Briefly, this product is produced by a typical NRPS assembly line of four subunits: PchD, PchE, PchF, and PchG. PchD activates salicylate, PchE and PchF successively integrate two l-cysteines into the growing peptide to form two thiazoline rings, and PchG then reduces the second thiazoline ring to thiazolidine before the release of mature pyochelin. The adenylation domain (A) in PchE selects and activates l-cysteine; aryl carrier protein (ArCP) and peptidyl carrier protein (PCP) connect and transfer salicylate and l-cysteine using phosphopantetheine (pPant) arms, respectively; the heterocyclization domain (Cy) condenses and cyclizes the two substrates to form a thiazoline ring; and the inserted epimerase (E) catalyzes the epimerization of an l-cysteinyl moiety to d-cysteinyl during thiazoline ring formation. The structure of PchE adopts an “H”-shaped head-to-tail dimeric architecture containing five connected catalytic domains.

In conformation 3, the PCP domain of chain A binds at the acceptor site of the Cy domain, with the hydroxyphenylthiazolinyl-pPant ligand observed, representing the post-condensation state. The A domain (complexed with Cys-AMP and Mg2+ ligands) adopts the adenylate-forming conformation. In addition to the dynamic domains, the Cy-Acore domains between two chains of conformation 3 have an r.m.s.d. of 0.566 Å. After completing the A domain, the Asub domain is interrupted by the E domain, a noncanonical epimerase that catalyzes the epimerization of l-cysteinyl to d-cysteinyl. The C-terminal PCP domain is clearly resolved in conformation 3 of PchE. Key catalytic residues interacting with hydroxyphenylthiazolinyl-pPant can be clearly recognized in the A chain of conformation 3. N368 can form a hydrogen bond with the pPant arm atom. Notably, D480 may form a complex hydrogen bond network with S472, T474, Q482, and Y114 to form polar contacts with the thiazoline ring atoms. Intriguingly, in the PCP post-condensation conformation, in which ArCP departs from the Cy domain, the tunnel adopts a similar conformation previously observed with both EpoB and BmdB. Similarly, the “Y” tunnel of PchE Cy is truncated at the side of ArCP by the residue F372.

>MDLPPDSRTALRDWLTEQLADLLGEPLADVRALADDDDLLGCGLDSIRLMYLQERLRARGSTLDFAQLAQRPCLGAWLDLLACADRLSAPATVALPTAQDRDQPFELSSVQQAYWLGRGAGEVLGNVSCHAFLEFRTRDVDPQRLAAAAECVRQRHPMLRARFLDGRQQILPTPPLSCFDLQDWRTLQVDEAERDWQALRDWRAHECLAVERGQVFLLGLVRMPGGEDRLWLSLDLLAADVESLRLLLAELGVAYLAPERLAEPPALHFADYLAHRAAQRAEAAARARDYWLERLPRLPDAPALPLACAPESIRQPRTRRLAFQLSAGESRRLERLAAQHGVTLSSVFGCAFALVLARWSESAEFLLNVPLFDRHADDPRIGEVIADFTTLLLLECRMQAGVSFAEAVKSFQRNLHGAIDHAAFPALEVLREARRQGQPRSAPVVFASNLGEEGFVPAAFRDAFGDLHDMLSQTPQVWLDHQLYRVGDGILLAWDSVVGLFPEGLPETMFEAYVGLLQRLCDSAWGQPADLPLPWAQQARRALLNGQPACATARTLHRDFFLRAAEAPDADALLYRDQRVTRGELAERALRIAGGLREAGVRPGDAVEVSLPRGPQQVAAVFGVLAAGACYVPLDIDQPPARRRLIEEAAGVCLAITEEDDPQALPPRLDVQRLLRGPALAAPVPLAPQASAYVIYTSGSTGVPKGVEVSHAAAINTIDALLDLLRVNASDRLLAVSALDFDLSVFDLFGGLGAGASLVLPAQEQARDAAAWAEAIQRHAVSLWNSAPALLEMALSLPASQADYRSLRAVLLSGDWVALDLPGRLRPRCAEGCRLHVLGGATEAGIWSNLQSVDTVPPHWRSIPYGRPLPGQAYRVVDTHGRDVPDLVVGELWIGGASLARGYRNDPELSARRFVHDAQGRWYRTGDRGRYWGDGTLEFLGRVDQQVKVRGQRIELGEVEAALCAQAGVESACAAVLGGGVASLGAVLVPRLAPRAEGSMDLPAAQPFAGLAEAEAVLTREILGALLEAPLELDDGLRRRWLDWLADSAASALPSLDEALRRLGWQAAGLTAMGNALRGLLAGEQAPAALLLDPWLAPQAVAARLPDGREALARLLEALPTPAAGERLRVAVLDTRAGLWLDQGMASLLRPGLELTLFERSRVLLDAAATRLPERIVVQALDDGLLPAEHLGRYDRVISFAALHAYEASREGLALAAALLRPQGRLLLVDLLCESPLALLGAALLDDRPLRLAELPSLLADLAAAGLAPRCLWRSERIALVEALAPGLGLDAAALQAGLEQRLPQAMRPERLWCLPSLPLNGNGKVDRRRLAESMTRALGECRHEPSAEEPLEAHEQALAECWEAVLKRPVRRREASFFSLGGDSLLATRLLAGIRERFGVRLGMADFYRQPTLAGLARHLQVQTVEIEETQLEEGVLHHHHHHLPSWSHPQFEK[2x]>VSRNISNNGIKFTAAFEGFRGTAYRATPNEKYLTIGYGSYGPHVEPGKTITPGQGLLLLNRDMAKAVAAVDAVAHHSLTQSQFDAVCDLVYNAGAGVIAAATGTGKALRSGDVATLRAKLALFINQN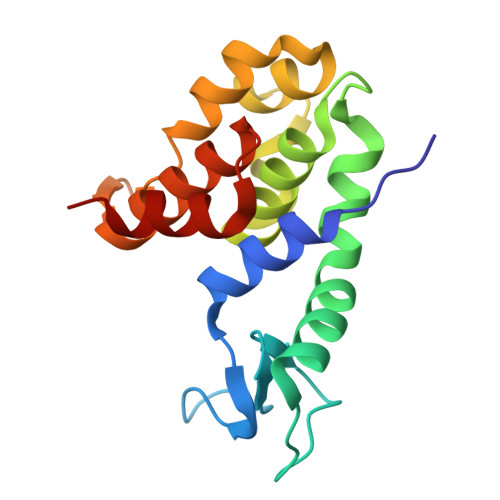GKPLLGLRRRTAGRLALFDGKPWQEAEAIGRAVK[3x]We apply the integrated NMR/EM approach to the dodecameric 12 × 39 kDa (468 kDa) large aminopeptidase enzyme TET2 from Pyrococcus horikoshii which forms a large hollow lumen encapsulating 12 peptidase active sites. The dodecameric assembly forms a tetrahedral structure with ca. 12 Å wide openings, one on each of the four tetrahedron faces, providing access to the ca. 50 Å wide catalytic lumen. NMR and EM thus provided structural information about TET2 on very different length scales, but neither of the two techniques by themselves allowed to determine the structure at the atomic scale, owing to the lack of long-range distance information in NMR, and the inability to build a robust model from the EM map.

Nonetheless, at 4.1 Å resolution, significantly better than the average of EM maps deposited over the last years, our EM data set is insufficient for de novo structure determination, highlighting the challenges that many EM data sets encounter. In step 3, a real-space structure refinement was applied in the XPLOR-NIH software, using the full Coulombic potential map, first at 8 Å, then at 6 Å and lastly at 4.1 Å resolution, and all NMR restraints, calculating the full dodecamer. We additionally explored a refinement with phenix.real_space_refine29 to refine these structures furthermore, and obtained an even slightly higher structure accuracy. In the general case, validation may comprise consistency checks against independent NMR data that have been left out from the calculation, or correlation with the EM map. In the case of TET2, a crystal structure was available, and the refined dodecameric structure is in excellent agreement with the crystal structure and the EM map. Possibly, interactions between residues in neighboring loops (residues 127–131) found to be in proximity in the EM map might stabilize the loop conformation, leading to a reduced but still visible density at cryogenic temperatures.

>MEVRNMVDYELLKKVVEAPGVSGYEFLGIRDVVIEEIKDYVDEVKVDKLGNVIAHKKGEGPKVMIAAHMDQIGLMVTHIEKNGFLRVAPIGGVDPKTLIAQRFKVWIDKGKFIYGVGASVPPHIQKPEDRKKAPDWDQIFIDIGAESKEEAEDMGVKIGTVITWDGRLERLGKHRFVSIAFDDRIAVYTILEVAKQLKDAKADVYFVATVQEEVGLRGARTSAFGIEPDYGFAIDVTIAADIPGTPEHKQVTHLGKGTAIKIMDRSVICHPTIVRWLEELAKKHEIPYQLEILLGGGTDAGAIHLTKAGVPTGALSVPARYIHSNTEVVDERDVDATVELMTKALENIHELKI[12x]>[2x]GIDPFTTRPSSDLTAFREHFAKAKHIAIITGAGVSAESGVPTFRGPGGFWRKWQAQDLATPEAFSRDPSLVWEFYHYRREVMRSKMPNPAHLAIAECEARLGQQGRSVVIITQNIDELHHRAGSKHVYEIHGSLFKTRCMSCGEVKANHKSPICPALDGKGAPDPNTKEARIPVELLPRCERKSCNGLLRPHVVWFGETLDSDILTAVERELEKCDL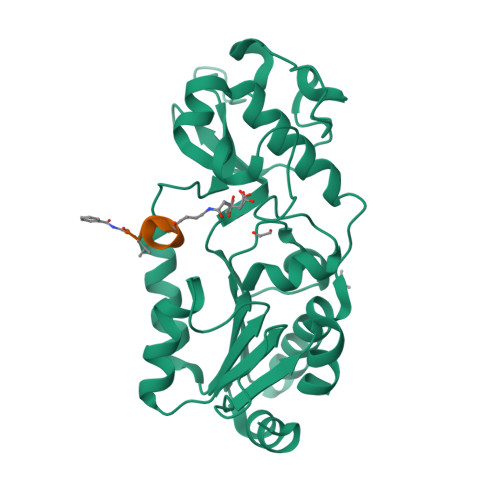CLVVGTSSIVYPAAMFAPQVASRGVPVAEFNMECTPATQRFKYHFEGPCGSTLPPALE;> XVLKEYGV>[6x]MSELFSERIPPQSIEAEQAVLGAVFLDPAALVPASEILIPEDFYRAAHQKIFHAMLRVADRGEPVDLVTVTAELAASEQLEEIGGVSYLSELADAVPTAANVEYYARIVEEKSVLRRLIRTATSIAQDGYTREDEIDVLLDEADR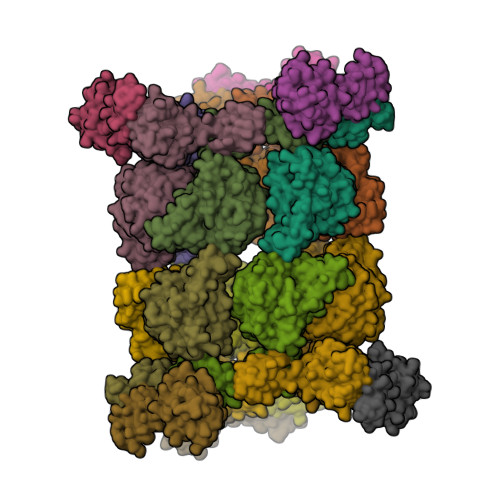KIMEVSQRKHSGAFKNIKDILVQTYDNIEMLHNRDGEITGIPTGFTELDRMTSGFQRSDLIIVAARPSVGKTAFALNIAQNVATKTNENVAIFSLEMSAQQLVMRMLCAEGNINAQNLRTGKLTPEDWGKLTMAMGSLSNAGIYIDDTPSIRVSDIRAKCRRLKQESGLGMIVIDYLQLIQGSGRSKENRQQEVSEISRSLKALARELEVPVIALSQLSRSVEQRQDKRPMMSDIRESGSIEQDADIVAFLYRDDYYNKDSENKNIIEIIIAKQRNGPVGTVQLAFIKEYNKFVNLERRFDEAQIPPGA;>KLLPAFQNAERLLLAHMMRSRDVALVVQERIGGRFNIEEHRALAAYIYAFYEEGHEADPGALISRIPGELQPLASELSLLLIADDVSEQELEDYIRHVLNRPKWLMLKVKEQEKTEAERRKDFLTAARIAKEMIEMKKMLSSS[3x]>MYTSSMTYESLYTKYRDDSAILKTEDYAHWTLPTVYADPDLREGKRVNVRRDYQSVGAVYVNTLSAKLAQVLFPANQAFFRIDSTGDAAQLAEAMGAESADLANGLAELENTAFRRIFLKSSYHQLVHAMKLLIITGNVLLYRDSNTGNMHAYSIRQYSVLRDGGGKVLDMVLKERTVISELPVEARIKYRNRKQDDCICLYTRIKRERRAVGEVFVVTQQLEDGLMLDNLEVYPEAICPFIPAVWNLVTGETYGRGLVEDYAGDLAKLSALSEALALYEIEACRVLHMAKPGSQIDVDSMAERESGAWVAGDPNGVAAYEAGDYNKIIALTQEIQSIAARLAPAFMYAQNQRNAERVTAEEIRQNAEEAELALGGVYSVIADTLHIPLAHILCWEVNQQFINELLSNGLTLSVLTGVAALSRSTDVNKLIQAAQSLSVILPVFQNTPRVDPEKILDMVLTGFGINTKDLYRTEEQLQALQAAQAPVTPDLANVAGTINETGL[12x];>MELLDAVNTCLTALGEARVTSTDTRHPSVALILQTLATKQKLLLERGWWFNTQDEEMFPDLLGRIPYPAASISVESLDGYNIYSKRNNFLFNNTCNTMYFTGPVCIRVTYNLDFEDLPESVATVITYRAARAVYVGDLGNDASVQDLVLNEQQAMLLVEEQHMRNKKHSTRRRRPWGKYQNALSG[12x]

Podophages that infect gram-negative bacteria, such as Pectobacterium pathogen ΦM1, encode tail assemblies too short to extend across the complex gram-negative cell wall. To overcome this, podophages encode a large protein complex (ejectosome) packaged inside the viral capsid and correspondingly ejected during infection to form a transient channel that spans the periplasmic space. Here, we report a near-complete atomic model of the bacteriophage ΦM1.

An adaptor assembly (gp52) interfaces with the portal and six tail fibers (trimeric gp47), each of which appears composed of long helical bundles much like phage T7, as well as adapts trimers of spike protein (gp39) which may be homologous to those in phage P22, another podophage, and 9NA, a siphovirus. The EP3 octamer adapts the locally 8-fold symmetric interface of the ejectosome to the 12-fold symmetric crown of the portal by intercalating the EP3 helix α-2 between the crown domains of adjacent portal monomers, forming contacts with the C-terminal portal helix. EP3 intercalates in a pattern in which two EP3 α-2 helices intercalate in the gaps between two adjacent portals, followed by an unoccupied gap. This results in four unoccupied portal crown domain gaps, and eight filled with the α-2 helices of the EP3 octamer. The C12 portal complex that sits in the locally C5 MCP environment results in a symmetrically incompatible interface that is best characterized by C1 symmetry. In our 3D classifications, we also identified two populations of particles in which ejectosome structures were aligned, but portal density was also rotated by ∼6° about the Z axis. This suggests that the ΦM1 portal may also exist as two discrete particle populations. Reconstruction of capsid dimers to low resolution reveals a probable interface forming between opposite and opposed adaptor proteins. Inspection of the dimer interface between symmetrized adaptor models auto-fit into the map suggested that this oligomerization likely forms due to formation of a putative reciprocal salt bridge network, forming between residues Arg25 and Asp23 of each chain of gp52. This hypothesis is tentative given the poor map resolution.> SLEIEELARFAVDEHNKKENALLEFVRVVKAKEQMFSWLDWEETMYYLTLEAKDGGKKKL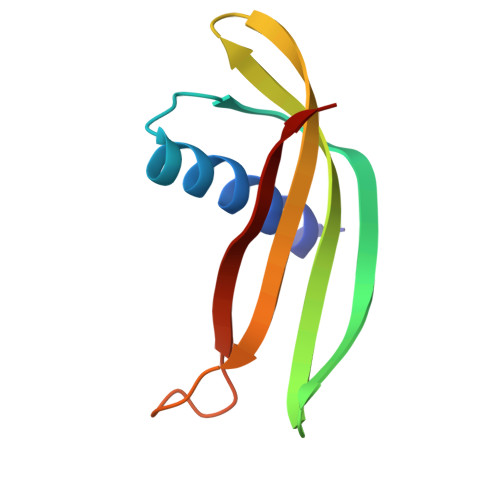YEAKVWVKPALLWSPHGNFKELQEFKPV>[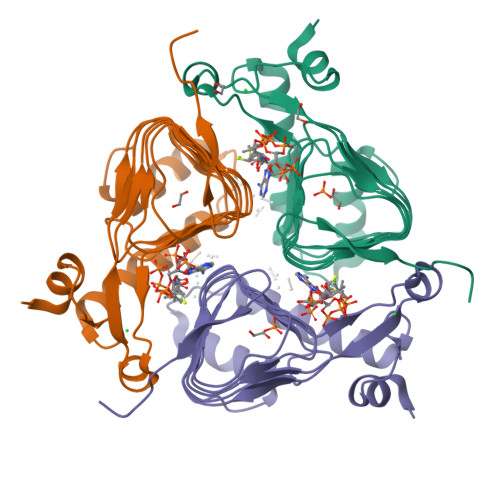3x]SNAMTEKEKMLAEKWYDANFDQYLINERARAKDICFELNHTRPSATNKRKELIDQLFQTTTDNVSISIPFDTDYGWNVKLGKNVYVNTNCYFMDGGQITIGDNVFIGPNCGFYTATHPLNFHHRNEGFEKAGPIHIGSNTWFGGHVAVLPGVTIGEGSVIGAGSVVTKDIPPHSLAVGNPCKVVRKIDNDLPSETLNDETIK>[2x]MMEFKKLVPYREALKLLLDDINEIEDTEKVPLREAVGRVLAEDIVTEFDIPPFDRAAVDGYAIRAEDTFQAREYNPIELTVIEEVPAGNVAKEEVTTGKAIKVLTGTRIPKGANAVIMQEMVKREGDKIYVLRPV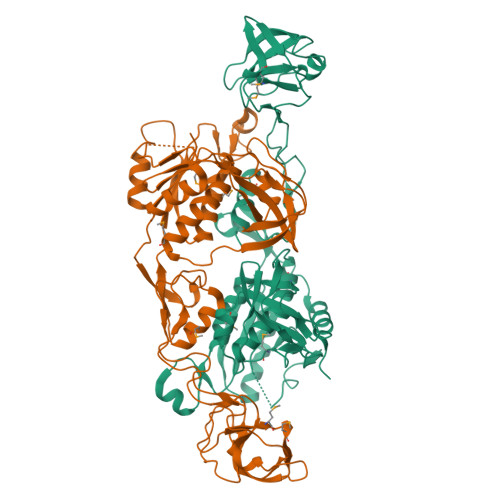APGQNIAFTGEDVKKGEVVLRKGTILRPQDVAMLKALGIKKVPVKVKPKVGIIITGSELIEEPSEEGFKEGKIVETNSIMLQGLVEKFFGEPILYGVLPDDESIIKETLEKAKNECDIVLITGGSAFGDKDYAHKFVNLLFHGTTIKPGRPFGYGEKVFIMSGYPVSVFAQFNLFVKHALAKMVGAQNYEVKVKAILQDDIPSQLGRYEFIKIYYENGIARVIKKKGSGILSSLLASNAYLEIPEDSEGYRRGEEVWITLY>[2x]G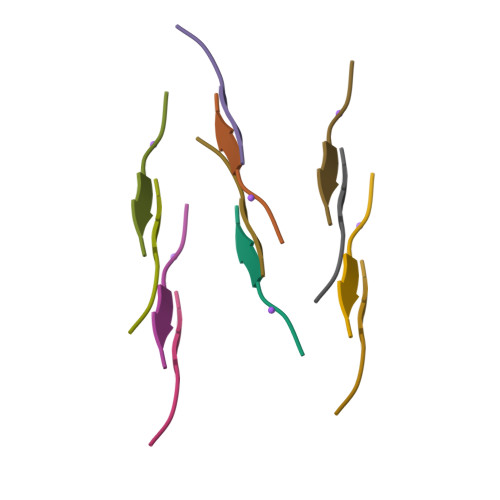GYLLG fos-choline-14 | C19 H43 N O4 P | 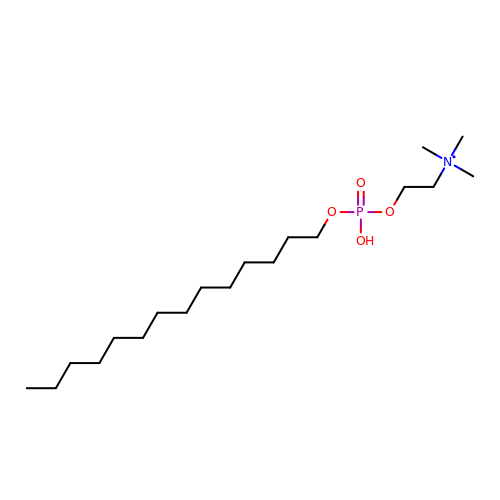JOPCRKJIQSCIFM-UHFFFAOYSA-N> MASSINPWILTGFADAEGSFGLYIINRNRGRIRYTTRLKFTITLHNKDKSILENIQSTWKVGIIANNGDNAVSLIVTRFEDLKVIIDHFEKYPLITQKLGDYKLFKQAFSVMENKEHLKENGIKELVRIKAKMNWGLTDELKKAFPGNISRERPLINKNIPNFKWLAGFTSGEGHFGVELIKNSRNSRVHVRLRFEIAQHVRDKNLMNSLITYLGCGYIYEQNYSERSWLRFSVSKFSDINDKIIPVFQENTLIGVKLEDFEDWCKVAKLIEEKKHLTESGLDEIKKIK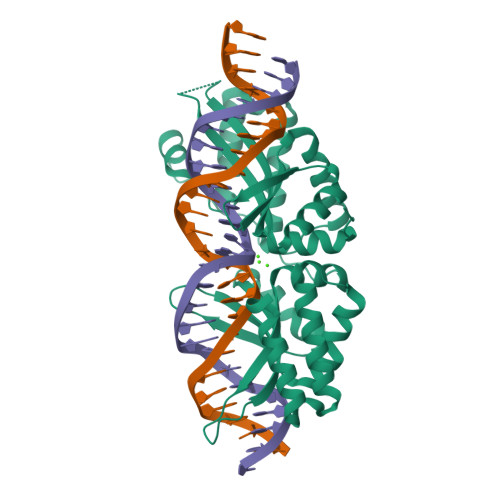LNMNKGR> ASRGSHHHHHHGASDDDDKEVVLLDFAAAGGELGWLTHPYGKGWDLMQNIMNDMPIYMYSVCNVMSGDQDNWLRTNWVYRGEAERIFIELKFTVRDCNSFPGGASSCKETFNLYYAESDLDYGTNFQKRLFTKIDTIAPDEITVSSDFEARHVKLNVEERSVGPLTRKGFYLAFQDIGACVA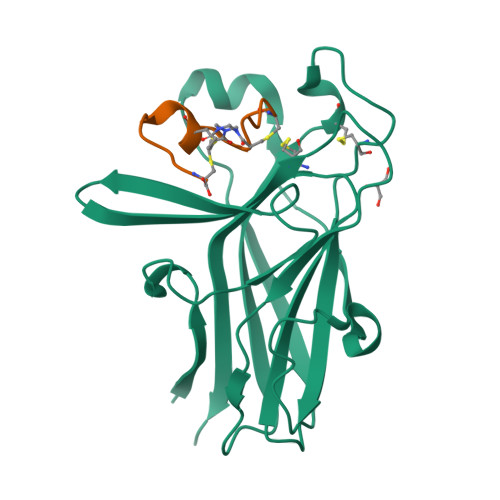LLSVRVYYKKC;> ARDCPLVNPLCLHPGWTC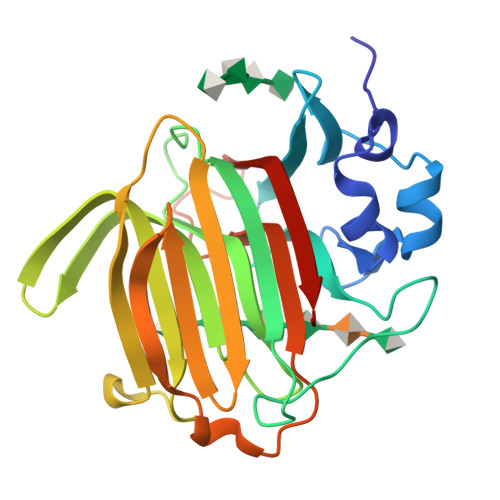> EFLTAVSSIDTFLPVLNEAKLQWPTSALAASSEELLGGYVGSQFYLQDGKYMQFQIAGSSNRCELRQMIPDGGSEIGWAVDDGTTHTATSSIVVPEQVDGVEEVTIMQINSGEAPQLRISWIRSKSLDGVAYEDFIMSTVRIGTGDSSDNFVKTHLADRTAGAMSFQIDVKDSKLTITVNGNVVVNGQDLSFWDGTDSCYFKAGAYNNNPTSESATARIKFAALAWVDHHHHHH>[2x]MASTAAETEKPEDHNDLVQLCNPHIAAMKEDILYHFSLSTSTHDFPAMFGDVKFVCVGGSPSRMKAFIKYVAMELGFAHPGADYPNICEGTDRYAMFKVGPVLSVSHGMGVPSIA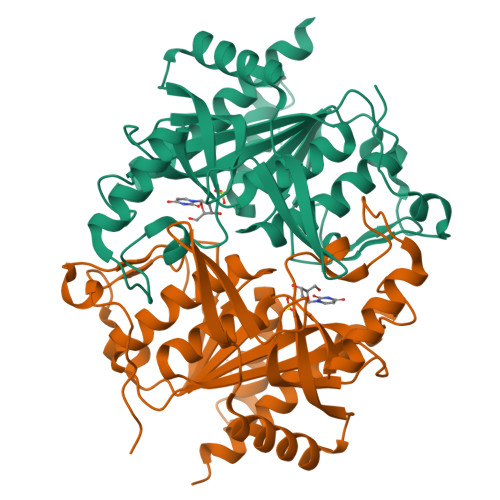IMLHELIKLLYHAHCSGVTLIRIGTSGGIGLEPGSVVITRQAVDPCFKPEFEQIVLGKREVRNTDLDEQLVQELARCSAELGEFPTVVGNTMCTLDFYEGQGRLDGALCSYTEKDKQDYLRAAYAAGIRNIEMEASVFAAMCNACGLRAAVVCVTLLNRLEGDQISSPHDVLAEYQQRPQRLVGQFIKKRLMQA> CCAA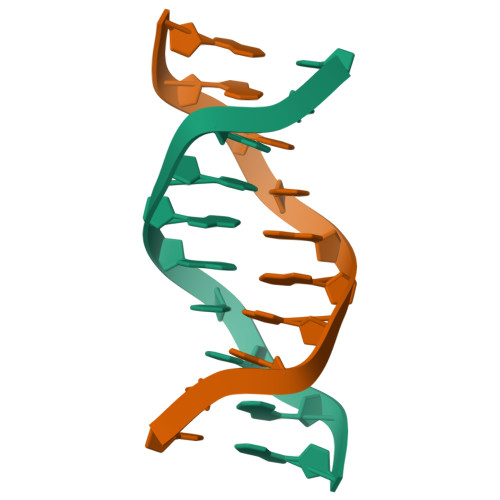IATTGG Human MLH1 (hMLH1) is a 756-amino-acid, 84 kDa protein that can be roughly divided into two halves: an N-terminal domain (NTD), where the ATPase activity resides, and a C-terminal domain (CTD), which is the site of dimerization with MLH1 paralogs. MLH1 homologs are conserved across all domains of life and are essential components of MMR. In higher eukaryotes, the MLH1 and PMS2 (postmeotic segregation increased 2) paralogs form a heterodimeric complex, MutLα. Once a lesion has been identified and isolated by the MutS mismatch-recognition complex, MutLα is recruited and, via its C-terminal endonuclease activity, generates nicks in the heteroduplex 3′ and 5′ to the mismatch that facilitate excision and replicative repair.

In this report, we present the X-ray crystal structure of a ternary Mg–ADP complex of the human MLH1 NTD domain determined to 2.30 Å resolution, which is the first report of a human MLH1 structure. Crystals of the hMLH1 NTD formed in space group P64 with one molecule in the asymmetric unit. The crystallized hMLH1 construct contained residues 1–340 of the full-length protein. The crystallographic model included amino-acid residues 3–85, 98–299 and 320–336. The ATPase domain (residues 25–207) contains the noncanonical, ATPase Bergerat fold, the core of which is composed of a four-stranded, antiparallel β-sheet (β1–β3 and β5) and three α-helices (αB–αD). In addition to the similarity observed in the overall structure between hLN40 and the MutL structure, we also observed the presence of an hLN40 crystallographic dimer similar to that observed in the E. coli MutL–Mg–ADP complex. However, in contrast to the prokaryotic structure, the hLN40 ATP-binding loop is partially disordered, possibly owing to crystal packing. Gly98 and Gly101 are positioned adjacent to the pyrophos­phate moiety of the bound ADP, permitting the close approach of ADP to the N-terminus of helix αD. Residues 301–320 in the hLN40 QTK loop are disordered; however, we can infer from MutL structures that Lys311 within the PTK motif should act as the conserved basic, γ-phosphate-sensing residue.

> GMSFVAGVIRRLDETVVNRIAAGEVIQRPANAIKEMIENCLDAKSTSIQVIVKEGGLKLIQIQDNGTGIRKEDLDIVCERFTTSKLQSFEDLASISTYGFRGEALASISHVAHVTITTKTADGKCAYRASYSDGKLKAPPKPCAGNQGTQITVEDLFYNIATRRKALKNPSEEYGKILEVVGRYSVHNAGISFSVKKQGETVADVRTLPNASTVDNIRSIFGNAVSRELIEIGCEDKTLAFKMNGYISNANYSVKKCIFLLFINHRLVESTSLRKAIETVYAAYLPKNTHPFLYLSLEISPQNVDVNVHPTKHEVHFLHEESILERVQQHIESKLLGSNSSRMYFTQT>SAD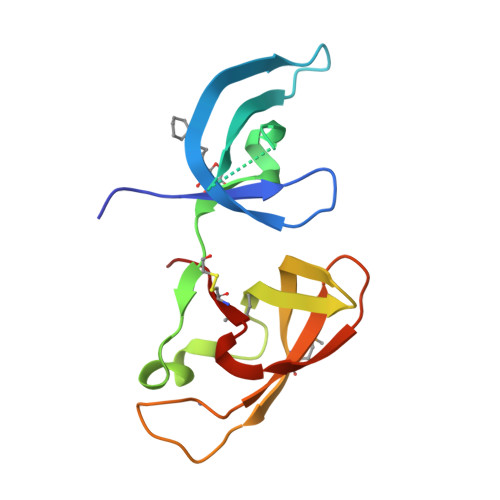LAFEAKSARDYAWYDVSSFLTYRVLRTGELEVRVRFSGFDNRHDEWVNVKTSVRERSIPVEPSECGRVNVGDLMLCFQEREDQALYCDGHVMNIKRGIHDHARCNCVFLVRYELDNTEESLGLERICRRPEE[2x]>[2x]MATLQDIGVSAGINILSAFVFFIIFAVLRLQPFNDRVYFSKWYLKGLRSSPARGGAFAQRFVNLDFRSYMKFLNWMPEALKMPEPELIDHAGLDSVVYLRIYWLGLKIFTPIAVLAWAVLVPVNWTNNTLEMAKQLRNVTSSDIDKLSVSNIPEYSMRFWTHIVMAYAFTIWTCYVLMKEYETIANMRLQFVASEARRPDQFTVLVRNVPPDADESVSELVEHFFLVNHPDHYLTHQVVCNANKLADLVKKKKKLQNWLDYYQLKYARNNSQRIMVKLGFLGLWGQKVDAIEHYIAEIDKISKEISKEREEVVNDPKAIMPAAFVSFKTRWAAAVCAQTQQTRNPTQWLTEWAPEPRDVFWSNLAIPYVSLTVRRLIMHVAFFFLTFFFIVPIAFVQSLATIEGIVKAAPFLKFIVDDKFMKSVIQGFLPGIALKLFLAFLPSILMIMSKFEGFTSISSLERRAAFRYYIFNLVNVFLASVIAGAAFEQLNSFLNQSANQIPKTIGVAIPMKATFFITYIMVDGWAGVAGEILMLKPLIMFHLKNAFLVKTDKDREEAMDPGSIGFNTGEPRIQLYFLLGLVYAPVTPMLLPFILVFFALAYIVYRHQIINVYNQEYESAAAFWPDVHGRVIAALVISQLLLMGLLGTKHAALAAPFLIALPVLTIGFHHFCKGRYEPAFIRYPLQEAMMKDTLETAREPNLNLKGYLQNAYVHPVFKGDEDDYDIDDKLGKFEDEAIIVPTKRQSRRNTPAPSIISGDDSPSLPFSGKLVGTGTLEVLFQ

Previously reported as putative ion channels sensitive to osmolality, a companion paper characterizes OSCA/TMEM63 family members as a novel family of MA ion channels conserved across eukaryotes. The structure of OSCA1.2 reveals a trapezoid-shaped homodimer with a two-fold symmetry axis perpendicular to the membrane. The bulk of the protein lies within the membrane; the transmembrane (TM) domain (TMD) of each monomer contains eleven TM helices. Topological similarities with mTMEM16A suggest that OSCA1.2 also has two pores and could conduct ions through a structurally analogous pathway lined by TM3-TM7.

We purified Arabidopsis thaliana OSCA1.2 expressed in HEK293F cells and determined cryo-EM reconstructions in lipidic nanodiscs and Lauryl Maltose Neopentyl Glycol (LMNG) detergent micelle with cholesteryl hemisuccinate (CHS) at 3.1 and 3.5 Å resolution, respectively. Structures of OSCA1.2 in nanodisc and LMNG were nearly identical (RMSD = 0.81 Å). A comparison of nanodisc-embedded and LMNG-solubilized structures hints at the positional flexibility of the subunits relative to each other while in the closed state.>MAAVTQPRGESKYDAIPGPLGPQSASLEGKVALVTGAGRGIGREMAMELGRRGCKVIVNYANSTESAEEVVAAIKKNGSDAACVKANVGVVEDIVRMFEEAVKIFGKLDIVCSNSGVVSFGHVKDVTPEEFDRVFTINTRGQFFVAREAYK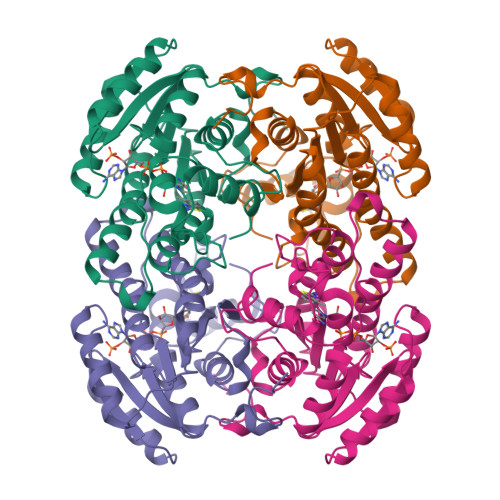HLEIGGRLILMGSITGQAKAVPKHAVYSGSKGAIETFARCMAIDMADKKITVNVVAPGGIKTDMYHAVCREYIPNGENLSNEEVDEYAAVQWSPLRRVGLPIDIARVVCFLASNDGGWVTGKVIGIDGGACM[2x]> UGGAGGGAAAAGUUAUCAGGCAUGCACCUGGUAGCUAGUCUUUAAACCAAUAGAUUGCAUCGGUUUAAAAGGCAAGACCGUCAAAUUGCGGGAAAGGGGUCAACAGCCGUUCAGUACCAAGUCUCAGGGGAAACUUUGAGAUGGCCUUGCAAAGGGUAUGGUAAUAAGCUGACGGACAUGGUCCUAACCACGCAGCCAAGUCCUAAGUCAACAGGAUGGUUCUGUUGAUAUGGAUGCAGUUCACAGACUAAAUGUCGGUCGGGGAAGAUGUAUU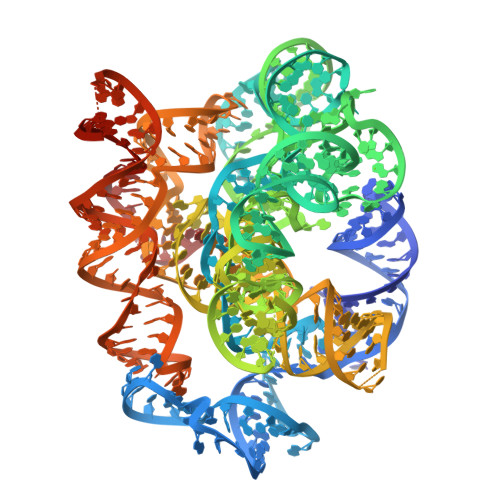CUUCUCAUAAGAUAUAGUCGGACCUCUCCUUAAUGGGAGCUAGCGGAUGAAGUGAUGCAACACUGGAGCCGCUGGGAACUAAUCAGUGAACCAUCCACUGAUUAGUUUUGGAGUACUCG> ALVIAFIGKNGAVMAGDMREITFEGEKPDREKLEKELYSGSIVTDEEMQKKAEEFGVKITVADCKEKVSERNGVLVGEVSSAEGGVVKKRRLYASAGNFAIAELINTEMTLTSQGKGSNFIAFGNEFTKQVANKCFKDNW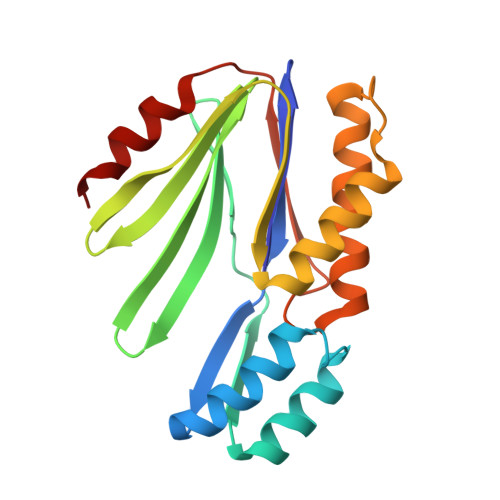TKKSNLQDAVKILILCMETVARKTASVSKQFMIVQTASNADVLKVVEKDRNS> QYAPQTQSGRTSIVHLFEWRWVDIALECERYLGPKGFGGVQVSPPNENIVVTNPSRPWWERYQPVSYKLCTRSGNENEFRDMVTRCNNVGVRIYVDAVINHMCGSGAAAGTGTTCGSYCNPGNREFPAVPYSAWDFNDGKCKTASGGIESYNDPYQVRDCQLVGLLDLALEKDYVRSMIADYLNKLIDIGVAGFRIDASKH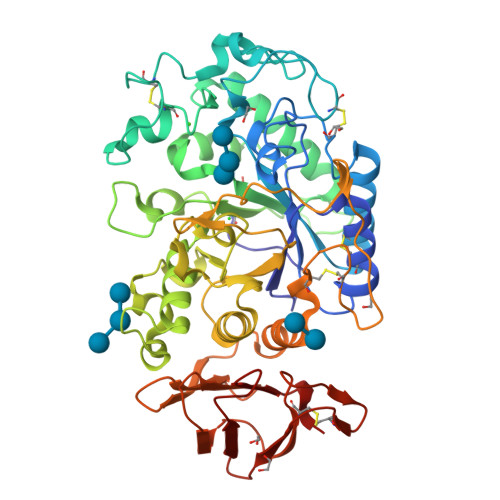MWPGDIKAVLDKLHNLNTNWFPAGSRPFIFQEVIDLGGEAIKSSEYFGNGRVTEFKYGAKLGTVVRKWSGEKMSYLKNWGEGWGFMPSDRALVFVDNHDNQRGHGAGGSSILTFWDARLYKIAVGFMLAHPYGFTRVMSSYRWARNFVNGEDVNDWIGPPNNNGVIKEVTINADTTCGNDWVCEHRWREIRNMVWFRNVVDGQPFANWWDNGSNQVAFGRGNRGFIVFNNDDWQLSSTLQTGLPGGTYCDVISGDKVGNSCTGIKVYVSSDGTAQFSISNSAEDPFIAIHAESKL The IM sub-complex comprises the ATP-binding cassette (ABC) transporter LptB2FGC, which extracts LPS from the IM and delivers it to the periplasmic components of the Lpt system. LptB2FGC is a type VI ABC transporter consisting of 5 subunits. The LptB cytoplasmic subunits form the nucleotide-binding domains (NBDs) that capture and hydrolyse ATP. LptF and LptG possess transmembrane helices that create a cavity and a translocation path for LPS, as well as a periplasmic β-jellyroll domain.

Three distinct conformations of LptB2FG, designated as LptB2FG-I, LptB2FG-II, and LptB2FG-III, were captured in our cryo-EM data and solved to resolutions of 3.34 Å, 3.26 Å, and 3.31 Å, respectively. The main difference between the three cryo-EM structures of LptB2FG is in the conformation of the β-jellyroll domain, which appears to perform a rigid body rotation motion with respect to the outer leaflet of the IM, transitioning from one conformational state to the other. The TMD and NBD domains of these three structures are essentially the same. In contrast to all the reported structures of LptB2FG determined by cryo-EM, our cryo-EM structures did not reveal any density consistent with the presence of LPS within the outward-facing cavity of the TMDs. This cavity has a volume of 5,473 Å3, approximately half the volume observed in the X-ray structure (10, 513 Å3), suggesting that the previously solved structure may represent an LPS-bound conformation. Intriguingly, our structures of LptB2FG exhibit an open V-shaped cleft at Interface 1, oriented toward the outer leaflet of the inner membrane, while Interface 2 remains entirely closed. This structural feature is expected to facilitate lipids entering the TMD domain of LptB2FGC via Interface 1. The distinctive structural attributes characterising our cryo-EM LptB2FG structures strongly suggest that we have captured the resting state, or substrate-free conformation, of this transporter. We identified four lipid molecules in LptB2FG-II and LptB2FG-III, likely originating from the nanodisc preparation used for sample reconstitution. These lipids were modelled as phosphatidylethanolamine (PE) moieties, arranged on the outer surface of the LptB2FG complex.

>[2x]MGSMATLKAQHLAKSYKGRQVVRDVSMSIDSGQIVGLLGPNGAGKTTCFYMIVGLVQADQGVVRIDEQNVTHLPMHGRARAGIGYLPQEASIFRKLSVSDNIMAILETRSDLDRNGRKEALEGLLQEFHIHHIRDNLGMSLSGGERRRVEIARALASAPKFILLDEPFAGVDPISVGDIKQIIHHLKAKGIGILITDHNVRETLDICETAYIVNDGQLIAEGDAESILANDLVKEVYLGHEFRLKLHHHHHH;> MGSMIVFRYLSREVLVTMSAVSAVLLVIIMSGRFIKYLAQAAQGLLDPGSLFLIMAFRIPGFLQLILPLGLFLGILLAYGRLYLESEMTVLSATGMSQKRLLGYTMAPALLVAILVAWLSLFLAPQGINQFALLLNKQDTLTEFDTLVPGRFQAMRDGTRVTYTEELSKDRGELAGIFISQKDLNSSNQERGISILVAEKGTQNIQADGSRYLILHNGYRYDGNPGQANYRAIQYDTYGVMLPKPEASSEVSERDAVPTADLFGSDNPRYQAELQWRLSTPLLVFVVTLLAVPLSRVNPRQGRFLKLLPAILLYMGYLALLIAVRGQLDKGKIPMAIGLWWVHGLFLAIGLLLFYWEPLRLKLASSRAGREVAHG;> MGSMVKLDRYIGVTVFVAILAVLGVILGLALLFAFIDELNDISASYGIGDALRFIFLTAPRRAYDMLPMAALIGCLVGLGTLASNSELTIMRAAGVSLSRIVWAVMKPMLVLMLAGILVGEYVAPWTENIAQSGRALAQGGGDSQSSKRGLWHRQGREYIHINAVQPNGVLYGVTRYRFDEQRGLESASFAKRARFETDHWQLEEVTTTLLHPREKRSEVVKLPTERWDAQLSPQLLNTVVMEPEALSISGLWQYIHYLADQGLNNNRYWLAFWTKVLQPLVTAALVLMAISFIFGPLRSVTLGQRIFTGVLVGFVFRIAQDLLGPSSLVFDFPPLLAVVIPASICALAGVWLLRRAG> MSNTISDRIVARSVIEAARFIQSWEDADPDSLTEDQVLAAAGFAARLHEGLQA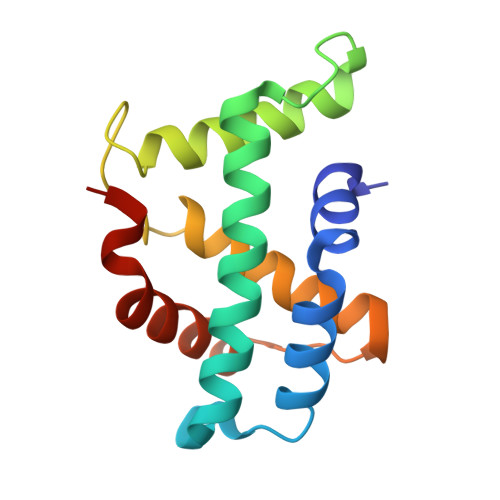TVLQRLVDESNHEEYREFKAWEEALLNADGRVASSPFADWGWWYRIANVMLATASQNVGVTWGSRVHGRLMAIFQDKFKQRYEEQA>MSDIFNSPQNKASILTALMKSTTGDVEDVLIPKRFRPAKDPLDSPQAAAQFLKDNKYRILRPRAIPTMVELETDAALPRLRQMVEDGKLKDTVSVPEGTTAFYPKYYPFHKPDHDEVGTFGAPDITLLKQLTFFLLENDFPTGPETLRQVREAIATLQYGSGSYSGQLNRLLAMKGVATGRNPNKTPKTVGYTNEQLAKLLEQTLPINTPKHEDPDLRWAPSWLINYTGDLSTDKSYLPHVTIKSSAGLPYIGKTKGDTTAEALVLADSFIRDLGRAATSADPEAGVKKTITDFWYLSCGLLFPKGERYTQVDWDKKTRNIWSAPYPTHLLLSMVSTPVMNESKLNITNTQTPSLYGFSPFHGGMDRIMTIIRDSLDNDEDLVMIYADNIYILQDNTWYSIDLEKGEANCTPQHMQAMMYYLLTRGWTNEDGSPRYNPTWATFAMNVAPSMVVDSSCLLMNLQLKTYGQGSGNAFTFLNNHLMSTIVVAEWVKAGKPNPMTKEFMDLEEKTGINFKIERELKNLRETIVEAVETAPQDGYLADGSDLPPIRPGKAVELDLLGWSAIYSRQMEMFVPVLENERLIASAAYPKGLENKALARKPGAEIAYQIVRYEAIRLVGGWNNPLLETAAKHMSLDKRKRLEVKGIDVTGFLDDWNNMSEFGGDLEGITLSEPLTNQTLVDINTPLDSFDPKARPQTPRSPKKTLDEVTTAITSGTYKDPKSAVWRLLDQRTKLRVSTLRDQALALKPASSSVDNWAEATEELAQ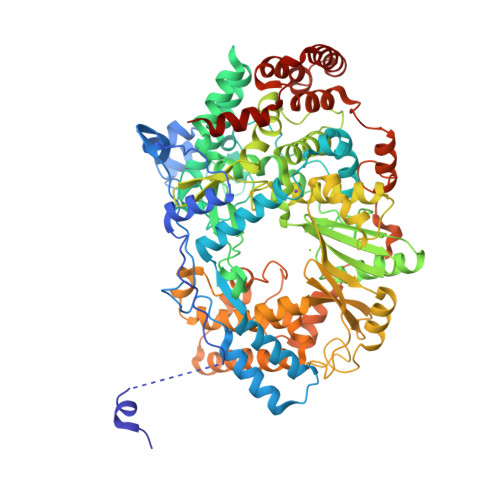QQQLLMKANNLLKSSLTETREALEKTGHHHHHH[5x]> GPLGSPEFMLPTNNNHRLISNSFSTYSIDTSRAYENYLTHWTEWKNNRIQEEQRDIAFQRLVSCLQNQETNLDLSELGLTTLPEIPPGIKSINISKNNLSLISPLPASLTQLNVSYNRLIELPALPQGLKLLNASHNQLITLPTLPISLKELHVSNNQLCSLPVLPELLETLDVSCNGLAVLPPLPFSLQEISAIGNLLSELPPLPHNIHSIWAIDNMLTDIPYLPENLRNGYFDINQISHIPESILNLRNECSIDISDNPLSSHALQSLQRLTSSPDYHGPQIYFSMSDGQQNTLHRPLADAVTAWFPENKQSDVSQIWHAFEHEEHANTFSAFLDRLSDTVSARNTSGFREQVAAWLEKLSASAELRQQSFAVAADATESCEDRVALTWNNLRKTLLVHQASEGLFDNDTGALLSLGREMFRLEILEDIARDKVRTLHFVDEIEVYLAFQTMLAEKLQLSTAVKEMRFYGVSGVTANDLRTAEAMVRSREENEFTDWFSLWGPWHAVLKRTEADRWAQAEEQKYEMLENEYPQRVADRLKASGLSGDADAEREAGAQ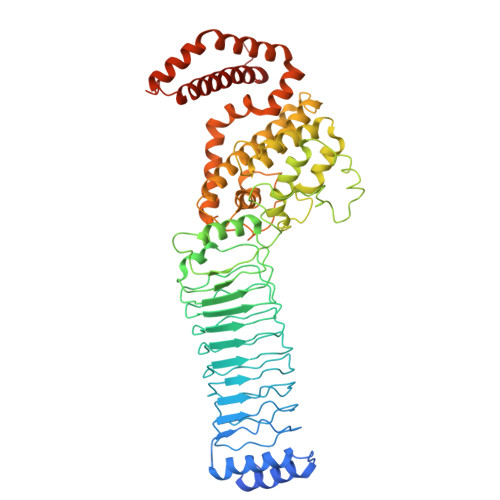VMRETEQQIYRQLTDEVLALRLPENGSQLHHS> LA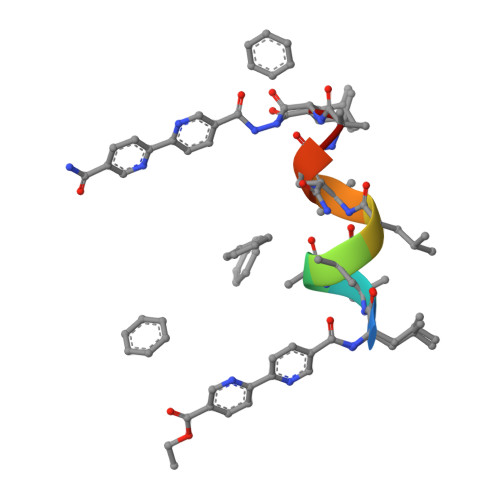AALAQAL> IEGYECQPIFLNVLEAIEPGVVCAGHDNNQPDSFAALLSSLNELGERQLVHVVKWAKALPGFRNLHVDDQMAVIQYSLMGLMVFAMGWRSFTNVNSRMLYFAPDLVFNEYRMHKSRM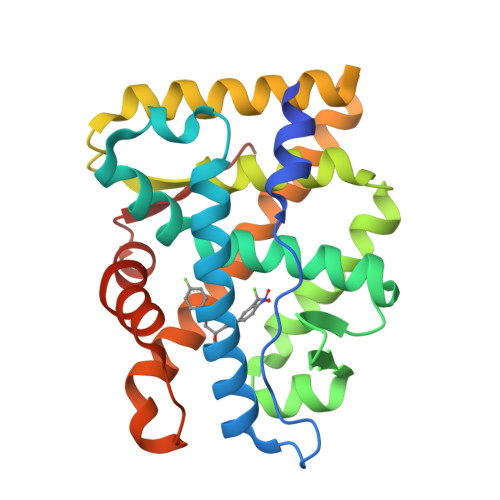YSQCVRMRHLSQEFGWLQITPQEFLCMKALLLFSIIPVDGLKNQKFFDELRMNYIKELDRIIACKRKNPTSCSRRFYQLTKLLDSVQPIARELHQFTFDLLIKSHMVSVDFPEMMAEIISVQVPKILSGKVKPIYFHTQ The unc-51-like kinase protein kinase complex (ULK1C) and the class III phosphatidylinositol (PI) 3-kinase complex I (PI3KC3-C1) are the most upstream and central players in the initiation of macroautophagy. FIP200 is the central scaffolding subunit of the ULK1 complex (ULK1C), which also contains the ULK1 (or ULK2) kinase itself, ATG13, and ATG101. PI3KC3-C1 contains one copy each of the lipid kinase VPS34, the pseudokinase VPS15, and the regulatory subunits BECN1 and ATG14. The two complexes coassemble through extensive contacts between the FIP200 scaffold subunit of ULK1C and the VPS15 pseudokinase subunit of PI3KC3-C1.

The ordered core of ULK1C was purified in a form consisting of the FIP200 N-terminal domain (1-640) and the ULK1 C-terminal microtubule-interacting and transport (MIT) domain (836-1059) fused with the ATG13 residues (363-517) responsible for binding to FIP200 and ULK1 ([Fig fig1]). Image processing and 3D reconstruction resulted in a cryo-EM density map with a local resolution of 3.35 Å in the best regions, including the FIP200:ATG13:ULK1 interface ([Fig figs1]). The structure confirmed the previous observation of a 2:1:1 FIP200:ATG13:ULK1 complex, while defining in residue-level detail how ULK1^MIT^ and ATG13^MIM^ bind to FIP200. The ULK1C core has dimensions of 180 × 130 × 90 Å, contains two molecules of FIP200^NTD^ and one molecule each of ULK1 and ATG13 ([Fig fig1]). FIP200 ^NTD^ forms a C-shaped dimer as seen at low resolution, which can now be described in detail with sequence assigned. The two arms of FIP200 consist of 120 Å-long bundles formed by three twisted helixes (81-495). The two arms are connected by an 80 Å-long dimerization domain (496-599) bent at nearly 90° to the arms, resulting in the C-shape. Cryo-EM density of for one copy of a ULK1^MIT^:ATG13^MIM^ heterodimer was observed on one “shoulder” of the FIP200 dimer. ULK1 binds directly to FIP200 via two main interfaces. The ATG13^MIM^ collaboratively binds to both FIP200 and ULK1^MIT^ ([Fig fig1], [Fig figs2]), consistent with the role of ATG13 in recruiting ULK1 downstream of FIP200.

>MKLYVFLVNTGTTLTFDTELTVQTVADLKHAIQSKYKIAIQHQVLVVNGGECMAADRRVCTYSAGTDTNPIFLFNKEMILCDRPPAIPKTTFSTENDMEIKVEESLMMPAVFHTVASRTQLALEMYEVAKKLCSFCEGLVHDEHLQHQGWAAIMANLEDCSNSYQKLLFKFESIYSNYLQSIEDIKLKLTHLGTAVSVMAKIPLLECLTRHSYRECLGRLDSLPEHEDSEKAEMKRSTELVLSPDMPRTTNESLLTSFPKSVEHVSPDTADAESGKEIRESCQSTVHQQDETTIDTKDGDLPFFNVSLLDWINVQDRPNDVESLVRKCFDSMSRLDPRIIRPFIAECRQTIAKLDNQNMKAIKGLEDRLYALDQMIASCGRLVNEQKELAQGFLANQKRAENLKDASVLPDLCLSHANQLMIMLQNHRKLLDIKQKCTTAKQELANNLHVRLKWCCFVMLHADQDGEKLQALLRLVIELLERVKIVEALSTVPQMYCLAVVEVVRRKMFIKHYREWAGALVKDGKRLYEAEKSKRESFGKLFRKSFLRNRLFRGLDSWPPSFCTQKPRKFDCELPDISLKDLQFLQSFCPSEVQPFLRVP[2x];> HTEILRGLRFTLLFVQHVLEIAALKGSASEAAGGPEYQLQESVVADQISLLSREWGFAEQLVLYLKVAELLSSGLQSAIDQIRAGKLCLSSTVKQVVRRLNELYKASVVSCQGLSLRLQRFFLDKQRLLDRIHSITAERLIFSHAVQMVQSAALDEMFQHREGCVPRYHKALLLLEGLQHMLSDQADIENVTKCKLCIERRLSAL;> DLGTFYREFQNPPQLSSLSIDIGAQSMAEDLDSLPEKLAVHEKNVREFDAFVETLQGSDEA>TVPGAXTV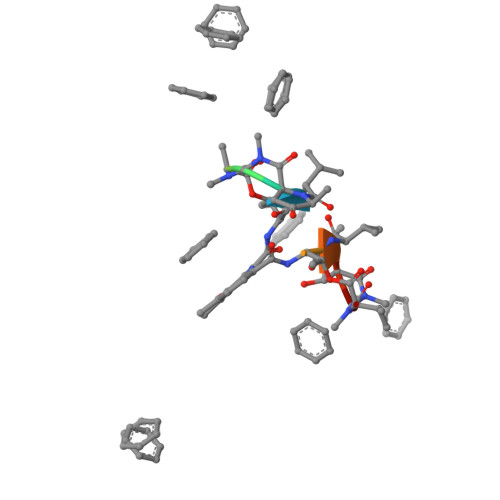PGV[2x]> MNVDLVFLFDGSMSLQPDEFQKILDFMKDVMKKLSNTSYQFAAVQFSTSYKTEFDFSDYVKWKDPDALLKHVKHMLLLTNTFGAINYVATEVFREELGARPDATKVLIIITDGEATDSGNIDAAKDIIRYIIGIGKHSQTKESQETLHKFASKPASEFVKI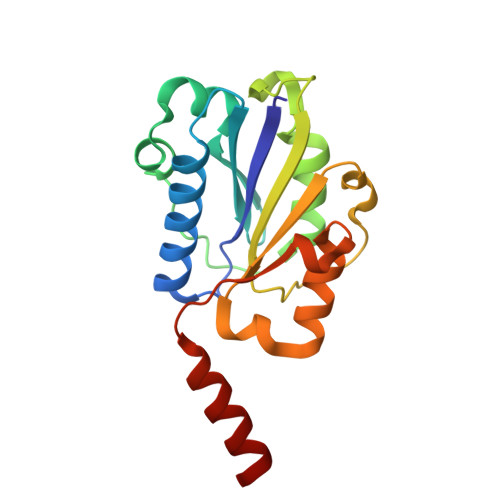LDTGEKLKDLFTELQKKIY> MKTVGEALKGRRERLGMTLTE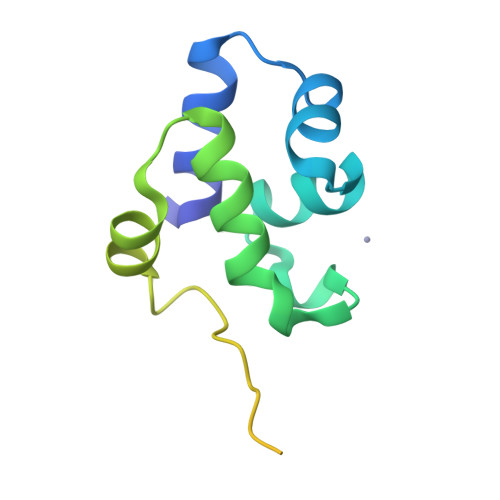LEQRTGIKREMLVHIENNEFDQLPNKNYSEGFIRKYASVVNIEPNQLIQAHQDEIPSNQAEWDEVITVFNNNKDLDYKSKSKEPIQLLVIMGITVLITLLLWIMLVLIF1-[(4-AMINO-2-METHYLPYRIMIDIN-5-YL)METHYL]-3-(2-{[HYDROXY(PHOSPHONOOXY)PHOSPHORYL]OXY}ETHYL)-2-METHYLPYRIDINIUM 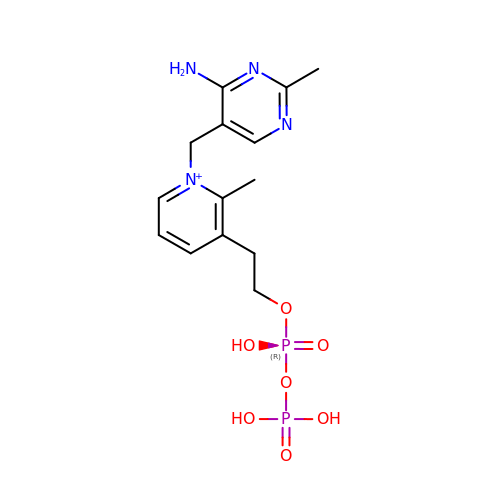| C14 H21 N4 O7 P2 | ZHKSTKOYQKNDSJ-UHFFFAOYSA-O> XY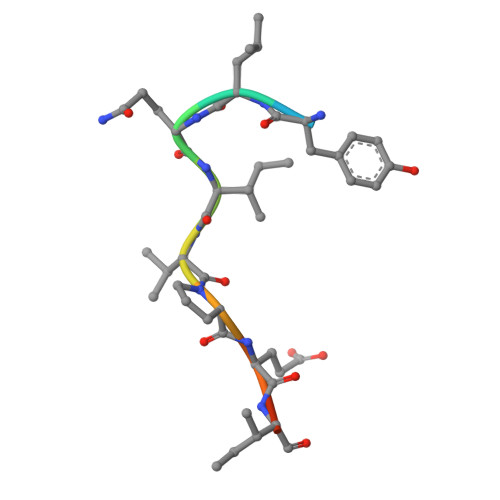LQIVPEIHK>MINNSFWQGKRVFVTGHTGFKGGWLSLWLQTMGATVKGYSLTAPTVPSLFETARVADGMQSEIGDIRDQNKLLESIREFQPEIVFHMAAQPLVRLSYSEPVETYSTNVMGTVYLLEAIRHVGGVKAVVNITSDKCYDNKEWIWGYRENEAMGGYDPYSNSKGCAELVTSSYRNSFFNPANYGQHGTAVATVRAGNVIGGGDWALDRIVPDILRAFEQSQPVIIRNPHAIRPWQHVLEPLSGYLLLAQKLYTDGAEYAEGWNFGPNDADATPVKNIVEQMVKYWGEG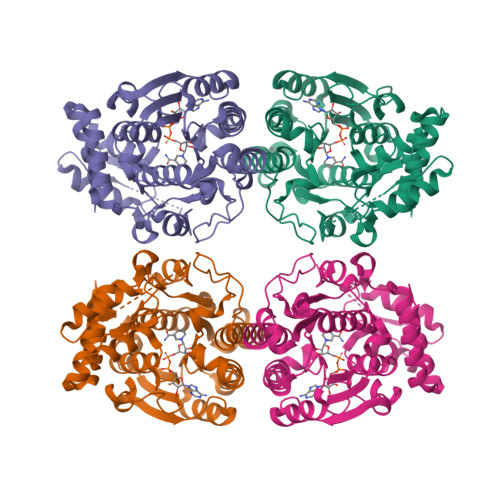ASWQLDGNAHPHEAHYLKLDCSKAKMQLGWHPRWNLNTTLEYIVGWHKNWLSGTDMHEYSITEINNYMNTK[4x]> GY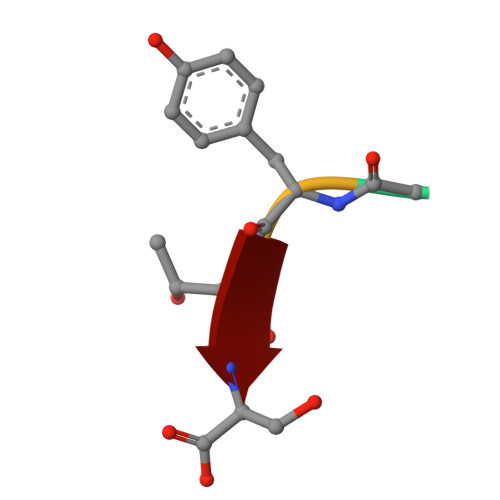TS>[3x]GSHMGLRGEYYNNMDFSRFQFVRIDPCIDFDWGEGTPDQSIGKDTYSVRWTGKVEPRYSETYTFYTVTDDGVRLWVDGVLLIDKWKSQSATEHSEQIYLEAGKKYDIKMEYYQHVRAASAKLMWSSKSQQKEIIPSSQLYPSDGPLPQKDVNGLSAEYYGDAELKDKRFTRIDDAINFNWDKDFPVGELKDGKFSVRWVGKIDTRYTEEYTFHTVANGGVRVWINNVLIIDNWQNQGKEAEN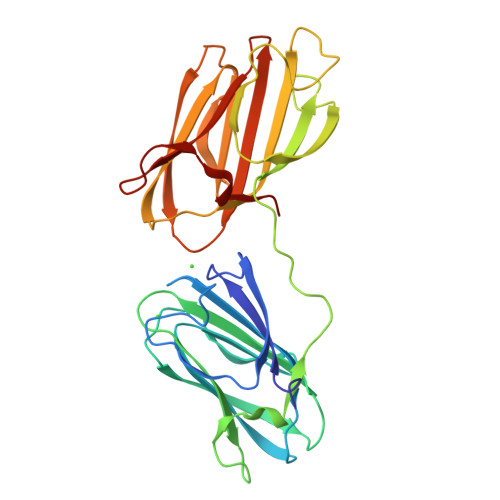SGKIELKAGRQYDIKVEYCNYGEPAFIKLLWSSQRQKKEVVPSKNLFAD> MSAIERIVKAAHLIDMCDIIREGNPSLRTVAEEVTFPLSDQEIILGEKMMQFLKHSQDPVMAEKMGLRGGVGLAAPQLDISKRIIAVLVPNIVEEGETPQEAYDLEAIMYNPKIVSHSVQDAA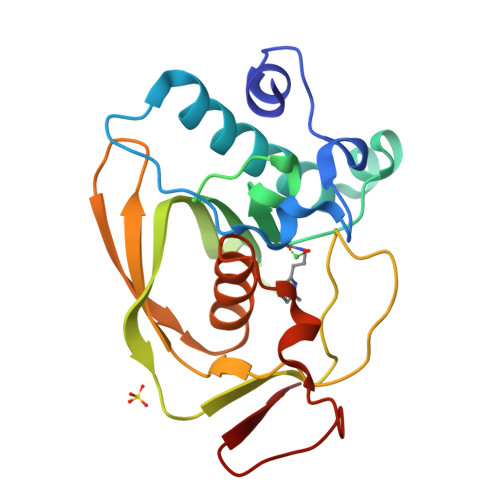LGEGEGCLSVDRNVPGYVVRHARVTVDYFDKDGEKHRIKLKGYNSIVVQHEIDHINGIMFYDRINEKDPFAVKDGLLILE>CGGACYCRI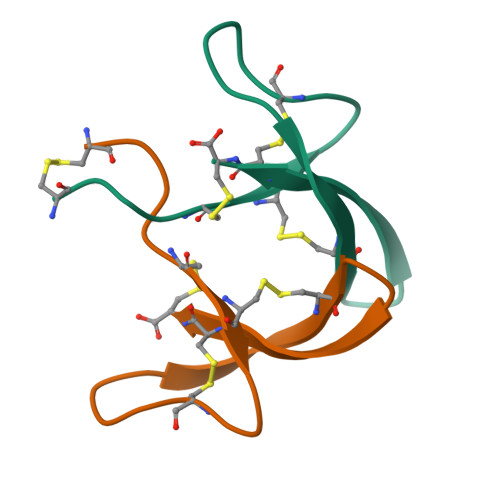PACIAGERRYGTCIYQGRLWAFCC[2x]> GDVVEAIEGAVARVADTISSGPTNSQAVPALTAVETGHTSQVVPGDTMQTRHVKNYHSRSESTIENFLSRSACVYMGEYYTTNTDETKRFASWTINARRMVQMRRKLEMFTYVRFDVEVTFVITSKQDQGTQLGQDMPPLTHQIMYIPPGGPIPKSTTDYAWQTSTNPSIFWTEGNAPPRMSIPFVSIGNAYSNFYDGWSHFSQNGVYGYNTLNNMGQLYMRHVNGPSPLPMTSIVRVYFKPKHVKAWVPRPPRLCQYKNASTVNFSSTNITDKRDSITHVPDTVKP;> SPSAEECGYSDRVRSITLGNSTITTQECANVVVAYGRWPEYLSDKEATAEDQPTQPDVATCRFYTLESVTWEKDSPGWWWKFPDALKDMGLFGQNMYYHYLGRAGYTIHVQCNASKFHQGCLLVVCVPEAEMGCSDVGGTVNEHAISEGEIAKKFSATATNGAHTVQSIVTNAGMGVGVGNLTIYPHQWVNLRTNNSATIVMPYINSVPMDNMFRHHNFTLMIIPFVSLDYSSDASTYVPITVTVAPMCAEYNGLRLATSLQ;> GLPVMNTPGSNQFLTSDDFQSPSAMPQFDVTPELDIPGEVKNLMEIAEVDSVVPVNNVVGKLDTMDIFRIPVQSGNHQSTQVFGFQVQPGLDSVFKHTLLGEILNYYAHWSGSVKLTFVFCGSAMATGKFLLAYSPPGANAPKTRKDAMLGTHVIWDVGLQSSCVLCIPWISQTHYRLVHQDEYTSAGNVTCWYQTGIVVPAGTPTLCSIMCFVSACNDFSVRLLKDTPFIEQSALLQ;> MGCVAETGDCGLPPDVPNAQPALEGRTSFPEDTVITYKCEESFVKIPGEKDSVICLKGSQWSDIEEFCNRSCEVPTRLNSASLKQPYITQNYFPVGTVVEYECRPGYRREPSLSPKLTCLQNLKWSTAVEFCKKKSCPNPGEIRNGQIDVPGGILFGATISFSCNTGYKLFGSTSSFCLISGSSVQWSDPLPECREIYCPAPPQIDNGIIQGERDHYGYRQSVTYACNKGFTMIGEHSIYCTVNNDEGEWSGPPPECRGGTKHHHHHH

Echoviruses, for which there are currently no approved vaccines or drugs, are responsible for a range of human diseases, for example echovirus 11 (E11) is a major cause of serious neonatal morbidity and mortality. Decay-accelerating factor (DAF, also known as CD55) is an attachment receptor for E11. The capsid consists of 60 identical protomers arranged with icosahedral symmetry and each protomer is composed of four capsid proteins, VP1–4, derived from the P1 polyprotein. DAF is one of the regulators of the complement system, inhibiting formation of the complement convertases in both the classical and alternative pathways.

In order to improve the density and characterize the interaction, symmetry expansion and selection of DAF occupied sites by variability analysis was performed. This analysis also indicated that the average number of DAF molecules bound per particle was ~20 and improved the density allowing, where there were contacts with the virus, some larger side chain orientations to be determined. SCRs 3 and 4 of DAF interact with E11 at the southern rim of the canyon via the VP2 EF and VP3 BC loops. We also observe an unexpected interaction between the N-linked glycan (residue 95 of DAF) and the VP2 BC loop of E11. The density for the glycan is not well enough defined to describe the interaction in detail, however it is clear that the BC loop of VP2 of E11 is involved, centered on Lys73. In the E6 pose, SCRs 2, 3 and 4 of one DAF molecule and two protomers of the capsid are involved in the interaction whilst in the E11 pose, only SCRs 3 and 4 and one protomer are directly involved, with the glycan of SCR1 interacting with a second protomeric unit. In support of this, it has been reported that a single amino acid substitution G162E in VP2 caused the loss of E11 affinity to DAF. Our structure confirms that a longer side chain at this position would clash with DAF in the E11 pose, so VP2 162 is a key residue controlling DAF binding pose.(1R,2R,3R,4S,5R)-4-amino-5-methoxycyclopentane-1,2,3-triol 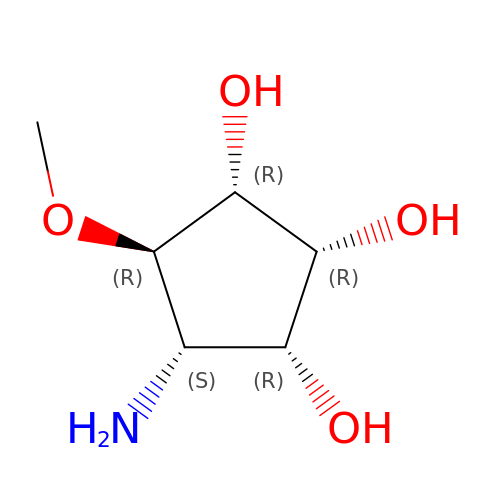| C6 H13 N O4 | NLCVJSNNNWJBCS-YDMGZANHSA-N> R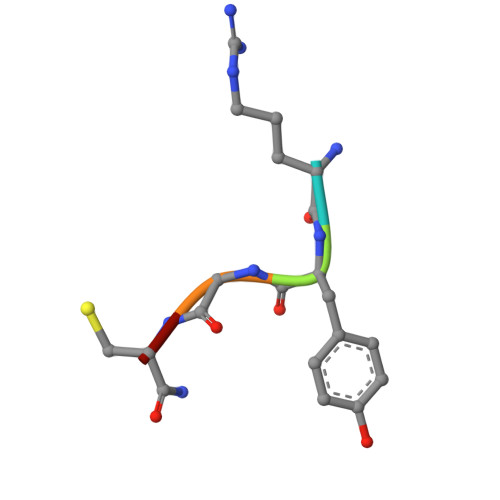YGCX>MRLFREIAANDPGPTGRMKNMKTFTTALATGVLALCPLAALADSSDPIVIPIHNWSSQIVMSNVVGQIFEEMGVAVEFVTTDSQAVYESVRLGDVTLELEVWEGAFGASFRAALEKGGIVDVGDHDAVTREDWWYPMWTKDACPGLPDWKALNDCAAVFATAETGDKGRYLDGPVDWLKHGKERVEALGMNFEVINAGSAAALWAEIGAAEADKRPVVVFNWTPNFAEAVWPGEFVEFPEWVDGCDKDPAVGPNPDALYDCGNPATGYLKKAAWEGMEAKWPDAYAVLTRISFTNPQIAEMAKLVDVDEMEPDEAAEAWLEANEDVWRPWLDGHHHHHH[2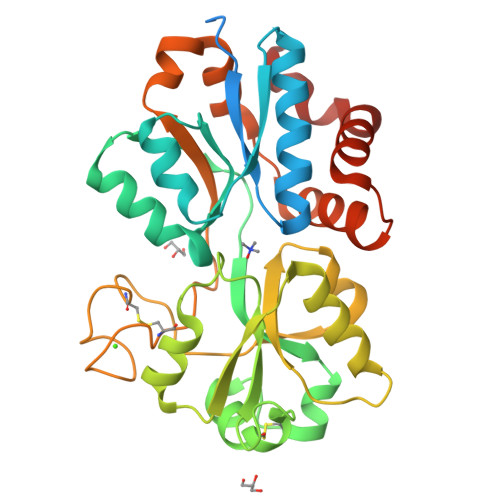x]> GSKTEGFMGRIRSVYPVASPQECNNMHLSTLMKCNHCDEVSWQTCDFLKATCEHCGTENLVIEGPTTCGYLPTNAVVKMPCPACQDPEIGPEHSVADYHNHSNIETRLRKGGRTRCFGGCVFAYVGCYNKRAYWVPRASADIGSGHTGITGDNVETLNEDLLEILSRERVNINIVGDFHLNEEVAIILASFSASTSAFIDTIKSLDYKSFKTIVESCGNYKVTKGKPVKGAWNIGQQRSVLTPLCGFPSQAAGVIRSIFARTLDAANHSIPDLQRAAVTILDGISEQSLRLVDAMVYTSDLLTNSVIIMAYVTGGLVQQTSQWLSNLLGTTVEKLRPIFEWIEAKLSAGVEFLKDAWEILKFLITGVFDIVKGQIQVASDNIKDCVKCFIDVVNKALEMCIDQVTIAGAKLRSLNLGEVF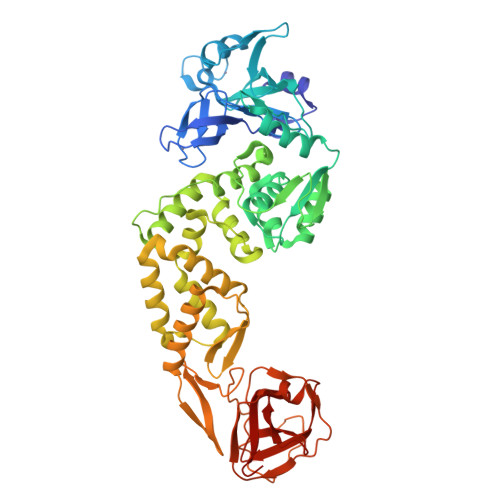IAQSKGLYRQCIRGKEQLQLLMPLKAPKEVTFLEGDSHDTVLTSEEVVLKNGELEALETPVDSFTNGAIVGTPVCVNGLMLLEIKDKEQYCALSPGLLATNNVFRLKGG> MDREEPAESECTLRALVEEYNGACKEAPKEMSKQFTDYNTFKRYTTSKKDHAPQMRLVYSVRKPWPISMTPSKEIPLVFNGTKLKDTILDLGESKRTRANIVVPDYWSKYGSQTSLEVVNAILYAEDLKVQRFFSTEWGEIRYGRMLPFRKPVQACPTIEEVNPASIPHTLLQVFCPQYTTLDSKRKAHMGAVEKLKRVMEPICKVQTQESAVHIARSLIDSNKKWLPTVVDHTPRTAEMAHFLCSKYHYVHTNTQDLSDTRSIDNLCGELVKRSLKCRCPKETLVANLDKITIQGRPMREVLADHDGELPYLGICRVAMGLSTHHTMKIRSTKFSILNSDHPRIEVKKVFSLSPDVQVTIPYRRFKGKAKVYFQNDQIQGYFSCTDRQIDEIKISAPKNAPLLEPLLDICYYGSFIEPGFEQTFGFYPAGKREFVDSFFMHHSKDHKAFLIHMGLDKDLSLPLSPELNWKEPALSKVCRVTELDSTVQPYTSATREFVLGETLNVYTQHENGLELLICPTEIRSTRGPLPPGTNLSGSEFIDIYQDPFSRAKSLLKSTILHAERCKEFVGNMLEEYQDPAETTVQSLVPINTWGKSAKRKLQEEITSDPDWHQCPRKRAKMSYLAIIAGSIQDRDKKQTNVPRAFMLRGSQIEYDMKATRGLVVDTTNRIIVGGETVLREGKGGPEGYVQT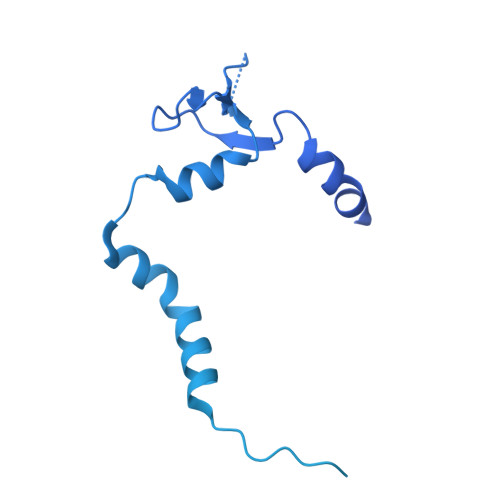GVFEEQPRCYLVDTPDHGLSMGLSRFCVHSQGRYFQYEKKISIWEETDNIKATIDSQRDLKRRRDIEEMVSKRARIV(1R,2S,3R,4R)-3-amino-4-(3-methylphenyl)cyclopentane-1,2-diol | C12 H17 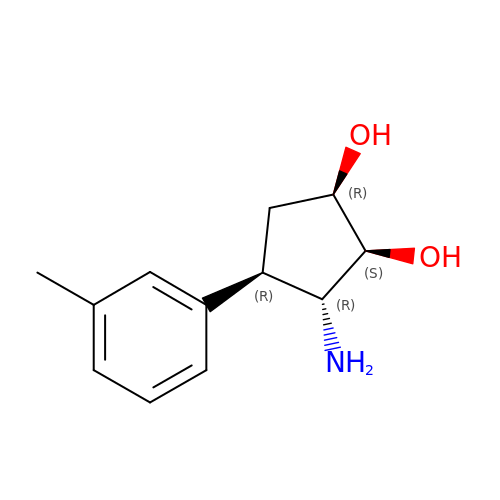N O2 | XKVIKQNAZKXWES-DDHJBXDOSA-N>[4x]MSISISYSTTYSGWTVADYLADWSAYFGD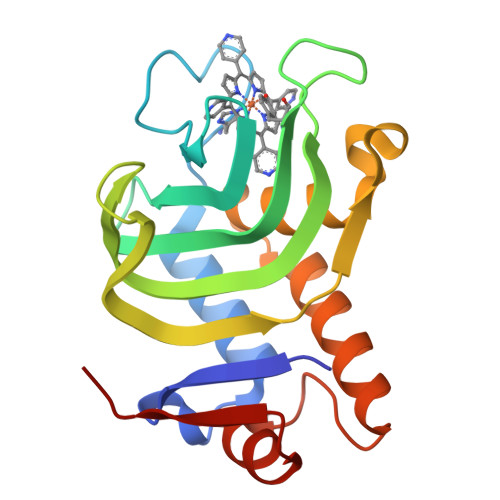VNHRPGQVVDGSNTGGFNPGPFDGSQYALKSTASDAAFIAGGDLHYTLFSNPSHTLWGKLDSIALGDTLTGGASSGGYALDSQEVSFSNLGLDSPIAQGRDGTVHKVVYGLMSGDSSALQGQIDALLKAVDPSLSINSTFDQLAAAGVAHATPAA> MAKKTSSKGKLPPGPSPLPVLGNLLQMDRKGLLRSFLRLREKYGDVFTVYLGSRPVVVLCGTDAIREALVDQAEAFSGRGKIAVVDPIFQGYGVIFANGERWRALRRFSLATMRDFGMGKRSVEERIQEEARCLVEELRKSKGALLDNTLLFHSITSNIICSIVFGKRFDYKDPVFLRLLDLFFQSF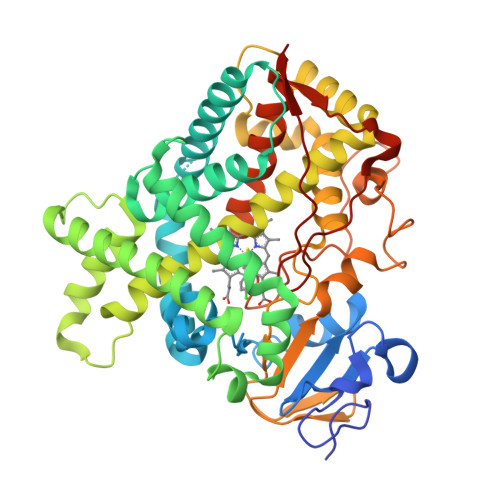SLISSFSSQVFELFPGFLKYFPGTHRQIYRNLQEINTFIGQSVEKHRATLDPSNPRDFIDVYLLRMEKDKSDPSSEFHHQNLILTVLSLFFAGTETTSTTLRYGFLLMLKYPHVTERVQKEIEQVIGSHRPPALDDRAKMPYTDAVIHEIQRLGDLIPFGVPHTVTKDTQFRGYVIPKNTEVFPVLSSALHDPRYFETPNTFNPGHFLDANGALKRNEGFMPHSLGKRICLGEGIARTELFLFFTTILQNFSIASPVPPEDIDLTPRESGVGNVPPSYQIRFLARHHHH> VKPLQVEPPEPVVAVALGASRQLTCRLACADRGASVQWRGLDTSLGAVQSDTGRSVLTVRNASLSAAGTRVCVGSCGGRTFQHTVQLLVYAFPNQLTVSPAALVPGDPEVACTAHKVTPVDPNALSFSLLVGGQELEGAQALGPEVQEEEEE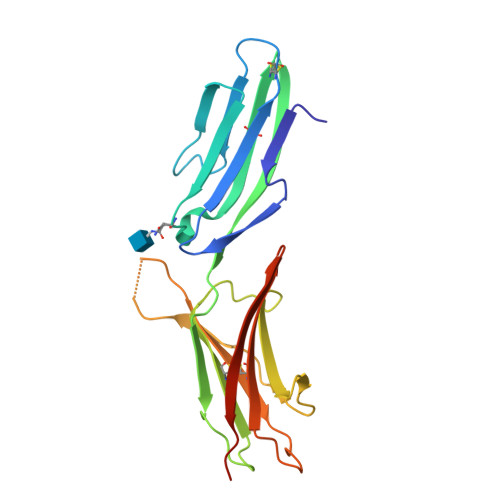PQGDEDVLFRVTERWRLPPLGTPVPPALYCQATMRLPGLELSHRQAIPVLHHHHHHH>[3x]MTETLPPVTESAVALQAEVTQRELFEFVLNDPLLASSLYINIALAGLSILLFVFMTRGLDDPRAKLIAVSTILVPVVSIASYTGLASGLTISVLEMPAGHFAEGSSVMLGGEEVDGVVTMWGRYLTWALSTPMILLALGLLAGSNATKLFTAITFDIAMCVTGLAAALT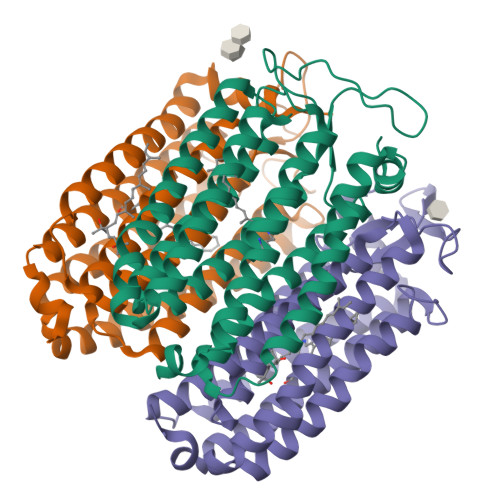TSSHLMRWFWYAISCACFIVVLYILLVEWAQDAKAAGTADIFSTLKLLTVVMWLGYPIVWALGVEGVAVLPVGYTSWAYSALDIVAKYIFAFLLLNYLTSNEGVVSGSILDVPSASGAPADD Epstein–Barr virus (EBV), a member of the Gammaherpesviridae, encodes the Bcl-2 homolog BHRF1, a potent inhibitor of Bcl-2-mediated apoptosis. EBV BHRF1 is a Bcl-2 homolog that potently inhibits host intrinsic apoptosis via direct inactivation of cellular proapoptotic Bcl-2 proteins Bak and Bim and selectively interacts with a subset of proapoptotic proteins (Bid, Puma, and Bax) to regulate apoptosis. Despite sharing very weak sequence identity with its cellular counterparts Bcl-2 (21.7%), Bcl-xL (17.9%), Bcl-w (18.4%), Mcl-1 (9.6%), Bfl-1/A1 (17.8%), and Bcl-B (21.5%), BHRF1 adopts the conserved alpha helical Bcl-2 fold comprising eight α-helices, with helices α2–α5 forming the canonical hydrophobic ligand-binding groove which provides the interaction site for the BH3-motif peptide. BHRF1 engages BH3 peptides using the canonical ligand-binding groove of its Bcl-2 fold and maintains a salt bridge between an Arg residue with a conserved Asp residue in the BH3 motif mimicking the canonical ionic interaction seen in host Bcl-2:BH3 motif complexes.

The structure of the BHRF1–BidBH3 complex was refined to a resolution of 2.78 Å, whereas the BHRF1–Puma BH3 complex was refined to 2.0 Å resolution. For the BHRF1–Bid BH3 complex, a clear and continuous electron density map was observed for BHRF1 residues 3–155 and BidBH3 motif residues 78–107. Bid BH3 is bound to BHRF1 via the canonical hydrophobic ligand-binding groove. The four canonical BH3 motif-defining residues from Bid, I86, L90, V93, and M97, engage four hydrophobic pockets of the canonical BHRF1 ligand-binding groove with an additional hydrophobic pocket occupied by a fifth hydrophobic residue, I83. Furthermore, these hydrophobic interactions are supplemented with two ionic interactions (salt bridges) between D95Bid and R100BHRF1, the hallmark of the pro-survival Bcl-2 interaction between a conserved arginine in the BH1 motif and aspartate of the BH3 motif, which is found in almost all pro-survival Bcl-2–BH3 complexes and R88Bid and E89BHRF1, as well as two hydrogen bonding interactions between D98Bid and G99BHRF1, and between R84Bid and E89BHRF1. In contrast to Bcl-xL–Bid BH3 and the previously determined structures of BHRF1–Bim and Bak BH3 motif complexes, Bid BH3 engages a fifth hydrophobic pocket of BHRF1. Residue I83Bid occupies a pocket formed by BHRF1 residues F72, T76, and V79, all residues highly conserved or conservatively substituted in BHRF1 variants. The use of a fifth hydrophobic pocket has previously been observed in several other viral Bcl-2–Bid BH3 complexes such as KsBcl-2 and the poxvirus variola virus F1L. A comparison of the BHRF1–Bid BH3 complex with KSHV KsBcl-2–Bid BH3 or VARV F1L–Bid BH3 shows that their mode of BH3 interaction is nearly identical, despite having significantly different affinities (110 nM, 20 nM, and 3220 nM toward Bid BH3, respectively).

>[5x]MGSHHHHHHSQDPMAYSTREILLALCIRDSRVHGNGTLHPVLELAARETPLRLSPEDTVVLRYHVLLEEIIERNSETFTETWNRFITHTEHVDLDFNSVFLEIFHRGDPSLGRALAWMAWCMHACRTLCCNQSTPYYVVDLSVRGMLEASEGLDGWIHQQGGWSTLIEDNIPG;>SESQEDIIRNIARHLAQVGDSMDRSIPPGLVNGL[5x]>ITGTSTVGVGRGVLGDQKNINTTYSTYYYLQDNTRGNGIFTYDAKYRTTLPGSLWADADNQFFASYDAPAVDAHYYAGVTYDYYKNVHNRLSYDGNNAAIRSSVHYSQGYNNAFWNGSQMVYGDGDGQTFIPLSGGIDVVAHELTHAVTDYTAGLIYQNESGAINEAISDIFGTLVEFYANKNPDWEIGEDVYTPGISGDSLRSMSD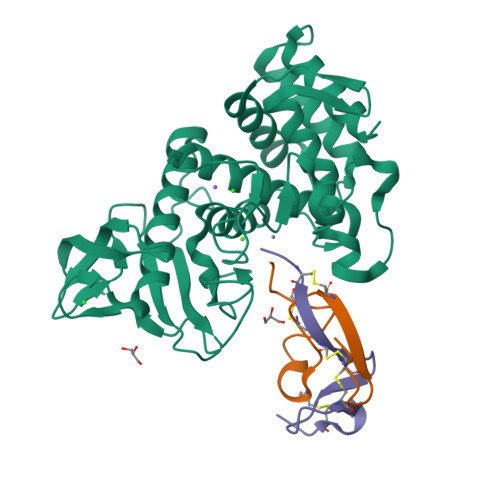PAKYGDPDHYSKRYTGTQDNGGVHINSGIINKAAYLISQGGTHYGVSVVGIGRDKLGKIFYRALTQYLTPTSNFSQLRAAAVQSATDLYGSTSQEVASVKQAFDAVGVK[2x];>GMSIVLICNGGHEYYECGGACDNVCADLHIQNKTNCPIIN[2x];>[2x]IRCNDKCYCEDGYARDVNGKCIPIKDCPKIRS> MSKPVKIGPWGGNGGSERDVQPKPIRMVSMTVSSGAIVDAIAFTYVGTDNVQHSSGIKWGGTGGTEDTI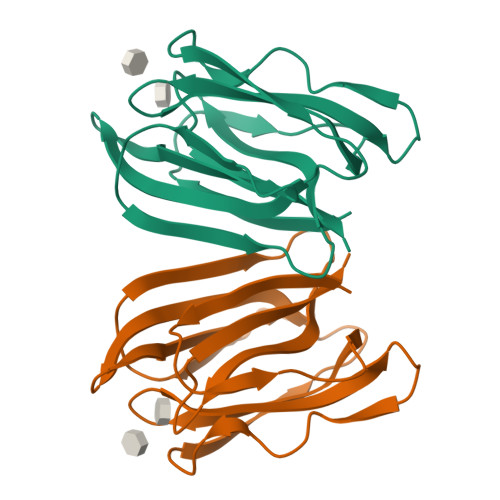NLDATNYVTEISGTVGKFGTDDIVTSLKIITSKGVTRTYGSGTGIPFRVPVLDGGKIAGFFGRAGAFLDAIGFYITP> GGKSEKLQEHLVAEQTSTFTEKEVYSSDKLIIKQVSPHTYVHVSFLDTDTFGKVACNGMIVISDGEAVVFDTPSTSNETSELLSFLEEEKLQVNAVVATHFHLDCLGGLEAFHARNIPSYAFKNTLSLASQHDFPQPQKGFSDELTLKVGTKAVFVHYFGEGHTQDNVIGYFPDDQVLFGGCLIKANGAGKGNLEDANVEAWPVTVNKISTAYPNLRLVIPGHGNWGDKTLLHYTETLFK

The class B MBLs are enzymes with the ability to hydrolyse virtually all β-lactam antibiotics, including carbapenems. Phylogenetically, MBLs can be grouped into three subclasses, B1 to B3.2 While enzymes belonging to subclasses B1 and B3 carry two Zn(II) binding sites (Zn1 and Zn2), B2 MBLs are mono-Zn(II) enzymes. In subclass B1, Zn1 is coordinated by three histidine residues (His/Gly116, His118 and His196), while the Zn2 binding site is coordinated by Asp120, Cys221 and His263.2,4–7 In B2 MBLs, the Zn1 binding site displays one altered residue (Asn116, His118 and His196), whereas the Zn2 site is identical to that of the subclass B1 MBLs. Here, we investigated three of these B1 MBLs,6 SHD-1, MYO-1 and ECV-1, in comparison with the clinically widespread enzyme NDM-1.

ECV-1 originated from Echinicola vietnamensis, which has previously been isolated from sea water. The structures of MYO-1 and ECV-1 were successfully solved by X-ray crystallography to 2.17 and 1.33 Å, respectively. The structure of ECV-1 was refined to an Rwork and Rfree of 0.16 and 0.19, respectively, with one molecule in the asymmetrical unit. In addition, MYO-1 and ECV-1 harboured in total three cysteine residues (positions 69, 121 and 221) within their active site. In contrast to the complex H-bond network in NDM-1 involving Ser69, Asp84, Lys121 and Ser262, we found different amino acids in MYO-1 (Cys69, Cys121, Gly262), ECV-1 (Cys69, Cys121, Gly262) and SHD-1 (Ala69, Arg121, Gly262). The lack of Lys121 or Arg121 in MYO-1 and ECV-1 was compensated for by an extensive network of water molecules. Interestingly, this loop was shortened by one residue at position 231 in both MYO-1 and ECV-1. At position 233, asparagine was present in both NDM-1 and ECV-1; however, we found tyrosine in MYO-1 and SHD-1. In addition, ECV-1 demonstrated high catalytic activity towards meropenem (65% compared with NDM-1), whereas imipenem, penicillins and cephalosporins were hydrolysed to a lower degree (∼10%–40%). ECV-1 and SHD-1 exhibited thermostabilities ∼3 and ∼8°C higher than MYO-1 and NDM-1.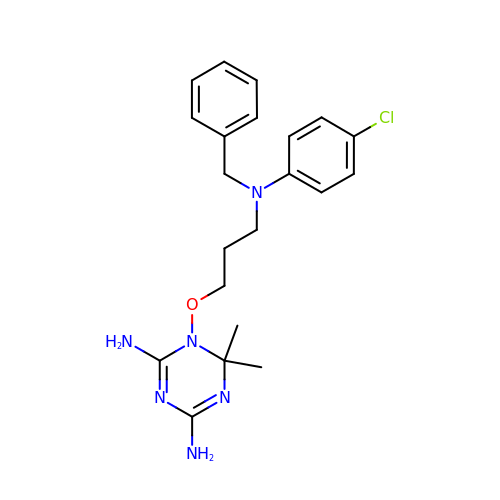1-[3-[(4-chlorophenyl)-(phenylmethyl)amino]propoxy]-6,6-dimethyl-1,3,5-triazine-2,4-diamine | C21 H27 Cl N6 O | XYRZUDPANKUJKS-UHFFFAOYSA-N> XAAAAAAQAVAGAAPVAA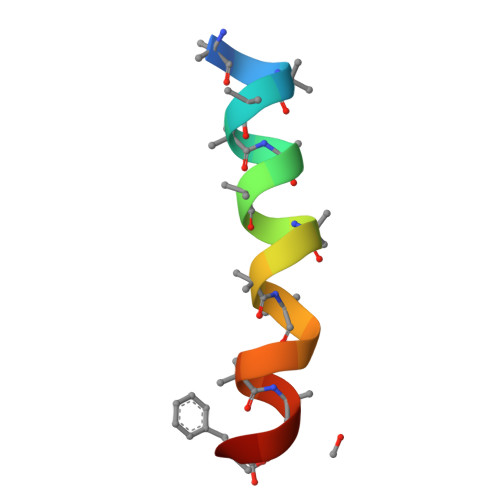QQF> EHLRLDNDQREKYIQEARNMGSTIRQPKLSNLSPSVIAQTNWKFVEGLLKECRNKTKRMLVEKMGREAVELGHGEVNITGVEENTLIASLCDLLERIWSHGLQVKQGKSALWSHLLHYQENRQRKLTSGSLSTSGILLDSERRKSDASAVMSPLRISLIQDMRHIQNIGEIKTDVGKARAWVRLSMEKKLLSRHLKQLLSDHELTKKLYKRYAFLRCDDEKEQFLYHLLSFNAVDYFCFTNVFTTILIPYHILIVPSKKLGGSMFTANPWICISG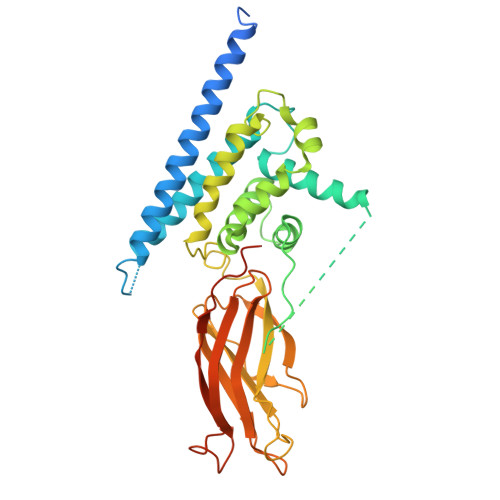ELGETQILQIPRNVLEMTFECQNLGKLTTVQIGHDNSGLYAKWLVECVMVRNEVTGHTYKFPCGRWLGKGMDDGSLERVLVGELLTSLPEVDERPCRTPPLQQSPSVIR2-[(2-methyl-3-nitrophenyl)amino]benzoic acid | C14 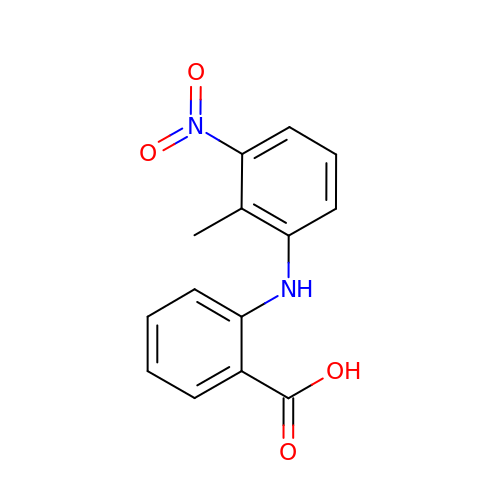H12 N2 O4 | HDSHJLYBOCCRCF-UHFFFAOYSA-N4-chloro-6-methylpyrimidin-2-amine | C5 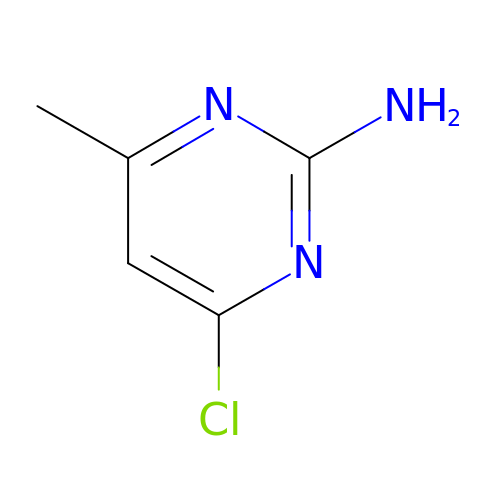H6 Cl N3 | NPTGVVKPLWFPPX-UHFFFAOYSA-N> SMAILFAVVARGTTILAKHAWCGGNFLEVTEQILAKIPSENNKLTYSHGNYLFHYICQDRIVYLCITDDDFERSRAFSFLNEVKKRFQTTYGSRAQTALPYAMNSEFSSVLAAQLKHHSENKSLDKVMETQAQVDELKGIMVRNIDLVAQRGERLE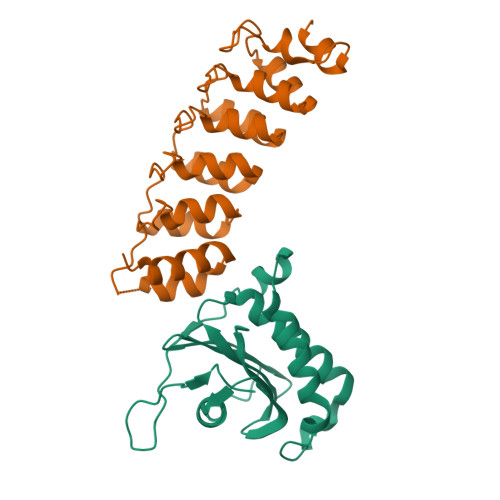LLIDKTENLVDSSVTFKTTSRNLARAMCMKNIK;> RQEETKKDYREVEKLLRAVADGDLEMVRYLLEWTEEDLEDAEDTVSAADPEFCHPLCQCPKCAPAQKRLAKVPASGLGVNVTSQDGSSPLHVAALHGRADLIPLLLKHGANAGARNADQAVPLHLACQQGHFQVVKCLLDSNAKPNKKDLSGNTPLIYACSGGHHELVALLLQHGASINASNNKGNTALHEAVIEKHVFVVELLLLHGASVQVLNKRQRTAVDCAEQNSKIMELLQVVPSCVASLDDVAETDRKEYVTVKIRKHHHHHH>AECSVD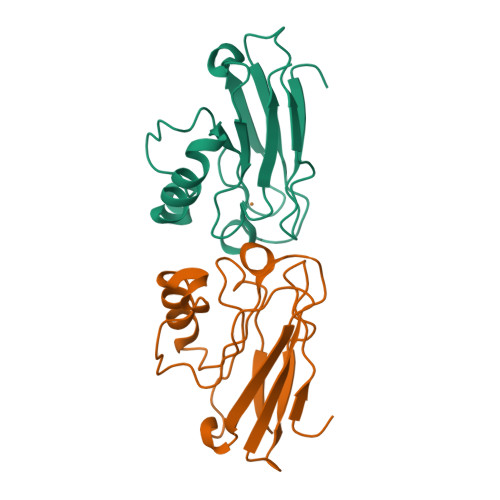IQGNDQMQFNTNAITVDKSCKQFTVNLSHPGNLPKNVMGHNWVLSTAADMQGVVTDGMASGLDKDYLKPDDSRVIAHTKLIGSGEKDSVTFDVSKLKEGEQYMFFCTAPGHSALMKGTLTLK[4x]N-[(4R)-6,8-dichloro-3,4-dihydro-2H-chromen-4-yl]-N'-(5-fluoro-1H-imidazo[4,5-b]pyridin-2-yl)propane-1,3-diamine | C18 H18 Cl2 F N5 O | 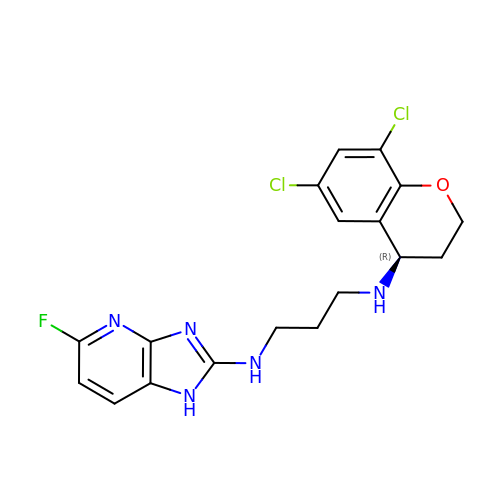YWDBMYZFLWAEHC-CYBMUJFWSA-N>LQPGIAQQWIQSKREDIVNQMTEACLNQSLDALLSRDLIMKEDYELVSTKPTRTSKVRQLLDTTDIQGEEFAKVIVQKLKDNKQMGLQPYPEILVVSRSPS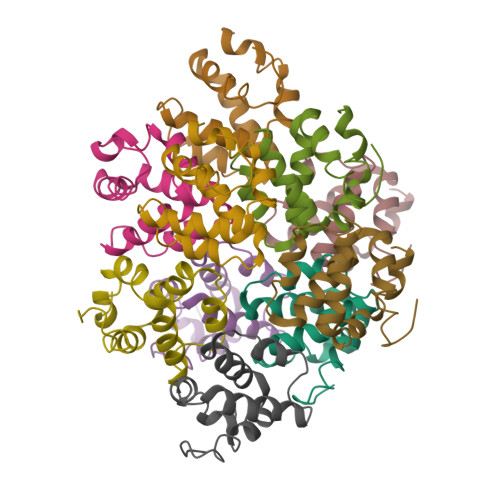LNLLQNKSM[10x]>GSHQKSFGGNYDRKLFAKLRKLRKSIADESNVPPYVVFNDATLIEMAEQMPITASEMLSVNGVGMRKLERFGKPFMALIR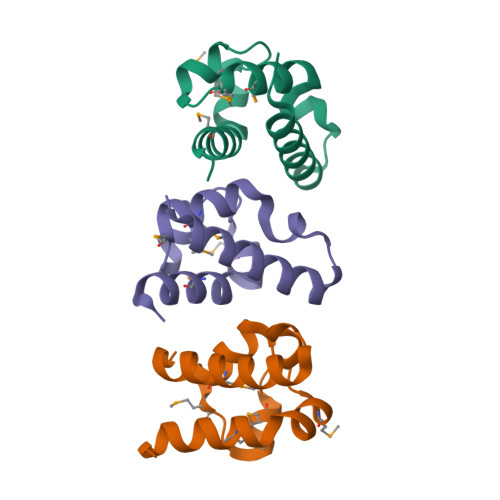AHVDGDDEE[3x]>[2x]STLKGALSVKFDVKCP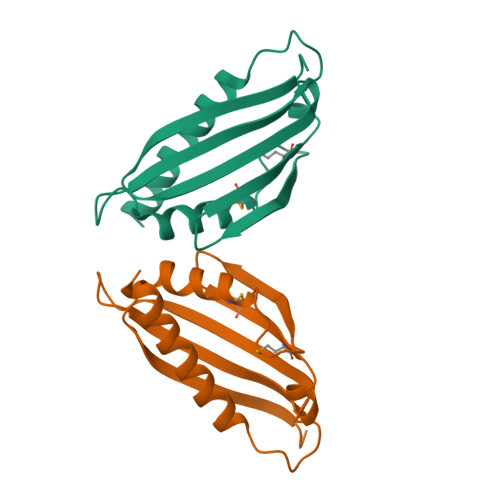ADKFFSAFVEDTNRPFEKNGKTEIEAVDLVKKTMTIQMSGSEIQKYFKTLKGSIAVTPIGVGDGSHVVWTFHFEKVHKDIDDPHSIIDESVKYFKKLDEAILNFKE> MQALRRGAAIPSRLLPRRDSWMSLAPFVAPNNAAAWRKLRDGAQEVQTVIERQSTPGKPQQIDWAKWESQIAHKDILNCLKTFYTNQVQILDRALGALETAKTPAPCEGAEKGWALFDAALSACAKSVEKSEELLSNGARALWVSCSNPPVWKVNTNEWLDSDQYWQAFVEKHHFYSQYQPGVVDPEA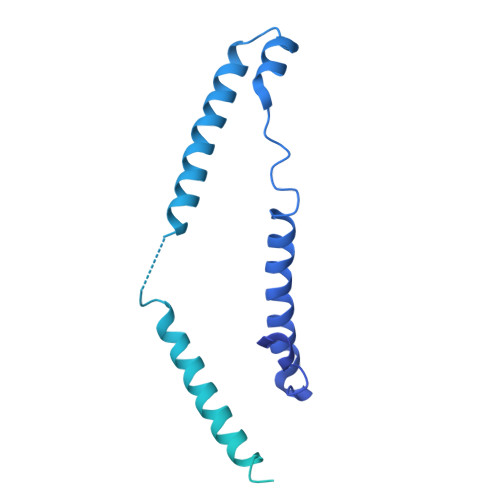PQEVEAFKQAWHSRMGKFNDRSDTPMLYAYMNELPSWEYYDLHRSAFLEHMTYFLVRTGGDFRFFPEMPPWQWLAHMENLRFKLLSVAQSRRSQLQLANLERERALDFLPVDVEHHGEEYTQKFLQYETELFQACAARLMGHFMFLCDPFIPVQSAEALSAVTRVDNGKGKLFSLGDDVNALFYLPEQQRRDVERPTQAVQTLLGHLEATGRPFNPCYSELLHVHAEVLEERGEHWLTAPGECVSQAFLRRLRTDDPAYEVYCSYFKEMYERFAGAKEVSMEDGRKRLATIEKNAQEEAAAYGLALKTMGSAELAHKAREGAAKLEQLRKAQEKAAGKSAQTVQENKM>[2x]MKLQVLPLSQEAFSAYGDVIETQ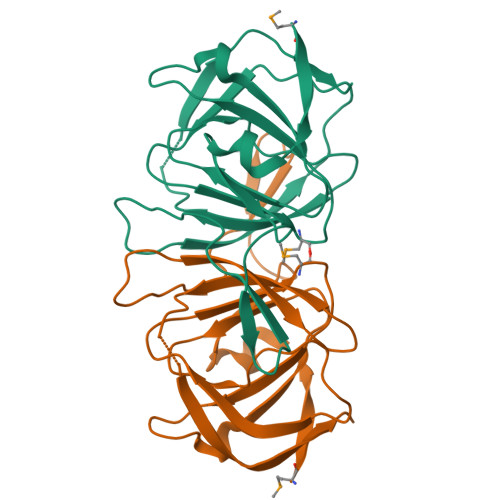QRDFFHINNGLVERYHDLALVEILEQDRTLISINRAQPANLPLTIHELERHPLGTQAFIPMKGEVFVVVVALGDDKPDLSTLRAFITNGEQGVNYHRNVWHHPLFAWQRVTDFLTIDRGGSDNCDVESIPEQELCFALEHHHHHH> MSQLSNQEKEYLISKALETEEGRVALAQAMANPIRVSLDYQGVGRKLLVVDPLPQGALPVYDKDVDAKAFVISKRGQVPDQVIEGDRIQVPTFEIVSYPQVRFSQVKERRFNVIDRAQQRAKADIMAVEDAEIFSLLEGAATAVNAVTISSGGLQRAALTKAFQEVEKHDLVVTK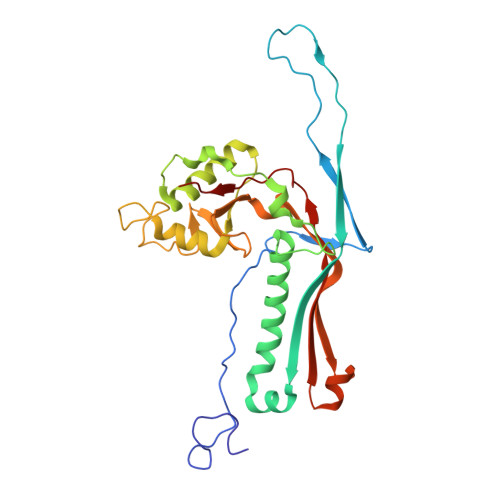IVMNASAFADIRAWGQNEFDPVTQHEVLQTGLFGHIWTADILISKKVPQNTVYVLADPEFVGVMPIRQDIQVIPADKPEELRLGWVIYEELGLAVVNSLAIAKIS> MSKYGPLGITNFITPYDLCILILIHAHCSQDNGISVPTAVFLRLISPTRPSLEWNPLLKDNSNLRSSSIVPPPVLPILDNIIRILLDDKDGNKIALTLMGYLEAINGLDSINRLMMDLEKNCLVNNYRSMKMRTTSTRRQMTRASFLGTFLSTCIRKYQIGDFEMRETIWINLQNFKTVFKHTPLWLRFKDNVHIQKVKNCLLANDEISVEDQQMVEFFQHFNNGNDADSKTMNEENYGTLISIQHLQSIVNRQIVNWLDNTEFNLMGQEETSSTYEEQSGLVFDLLDTLSLNDATKFPLIFILKYLEAIKENSYQTALDSLHNYFDYKSTGNSQNYFHISLLSLATFHSSFNECDAAINSFEEATRIARENKDMETLNLIMIWIINFIEVHPEYANRFYITVEQIIKYLKNSSDVEDANIFSNAYKFETLLSMVKESKTAEVSSSLLKFMAITLQNVPSQNFDLFQSLVSYEVKFWKELGYESISDVYEKFLSKTSSSSLRNYDSSIINQDIKVAFKALEEDDFLKVKQYLLKSESLELDYDQKINLKYLRVKYLVKIGDYDLSMRLINQYVKECCEEVADSNWRFKFEIESINVLLLSDVGIRSLPKIIKLIDEYKEIG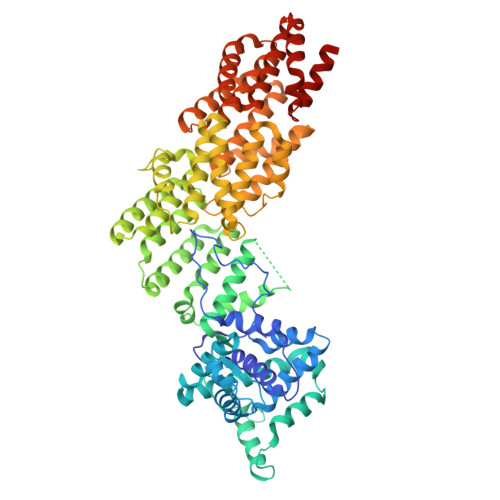NPLRCVILLLKLCEVLIQVGKSMEAECLISCNLSTILEFPFVRKKTDELLESLSVEEDRDVQMT>GIDPFTMTTARDIMNAGVTCVGEHET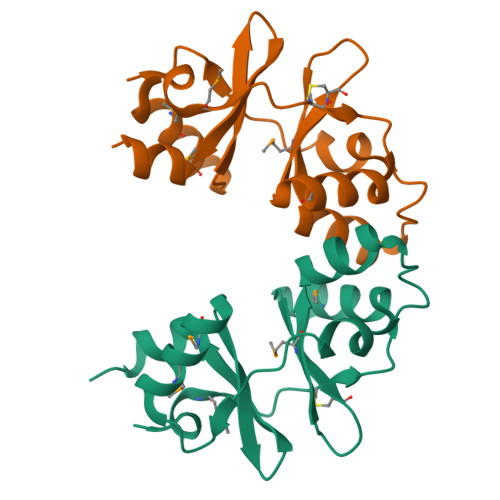LTAAAQYMREHDIGALPICGDDDRLHGMLTDRDIVIKGLAAGLDPNTATAGELARDSIYYVDANASIQEMLNVMEEHQVRRVPVISEHRLVGIVTEADIARHLPEHA[2x]>[2x]MLTIDYNSYRTTTPYGKRVRFLVLHY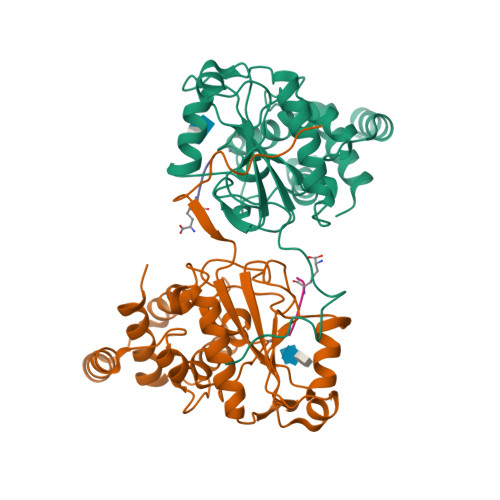TALDFAASVKALTTGAASAHYLIPAPHDPSYKAAGFKGQRIFNLVAEEDRAWHAGVSGWARRDNLNDTSIGIEIVNLARDDDGVFTFPDYERSQINALKQLAKNILQRYPDMTPKNVVGHSDIAVGRKSDPGPKLPWKELYEAGIGAWYDDATRDRYREGFERDGLPPRADLLEAFRLYGYALPATVDDAYFASLLRAFQMHFRPENYDGALDVETAAILYALNEKYPA;>[2x]AEKA>[2x]LALMSAAKLPKSFVWGYATAAYQIEGSPDKDGREPSIWDTFCKAPGKIADGSSGD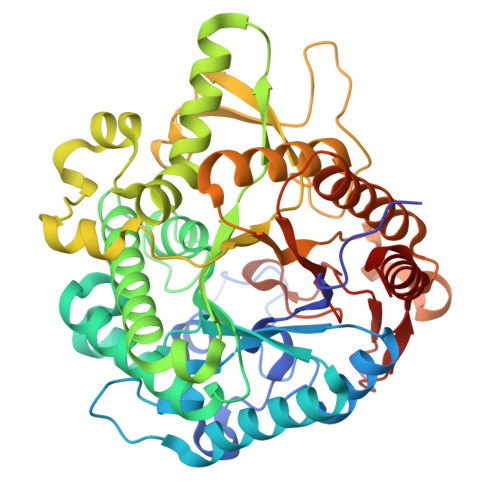VATDSYNRWREDVQLLKSYGVKAYRFSLSWSRIIPKGGRSDPVNGAGIKHYRTLIEELVKEGITPFVTLYHWDLPQALDDRYGGWLNKEEAIQDFTNYAKLCFESFGDLVQNWITFNEPWVISVMGYGNGIFAPGHVSNTEPWIVSHHIILAHAHAVKLYRDEFKEKQGGQIGITLDSHWLIPYDDTDASKEATLRAMEFKLGRFANPIYKGEYPPRIKKILGDRLPEFTPEEIELVKGSSDFFGLNTYTTHLVQDGGSDELAGFVKTGHTRADGTQLGTQSDMGWLQTYGPGFRWLLNYLWKAYDKPVYVTENGFPVKGENDLPVEQAVDDTDRQAYYRDYTEALLQAVTEDGADVRGYFGWSLLDNFEWAEGYKVRFGVTHVDYETQKRTPKKSAEFLSRWFKEHIEE>[2x]MASATIPAPAPRKMERAEGPASVLAIG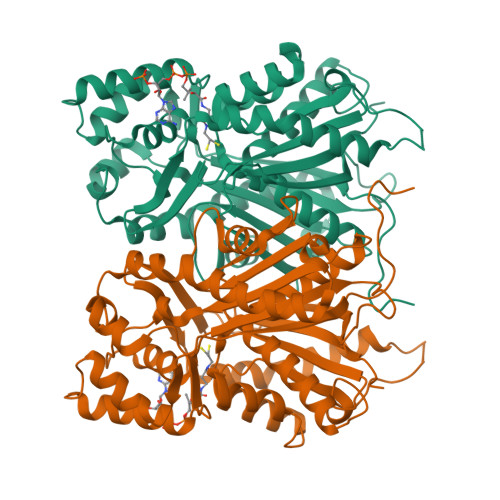TAVPPNVVYQKDYPDFYFGVTNSNHKTELKDKFQRMCDKSCVSKRHLYLTEEILKANPSLCAYWEPSLDLRQDIVVVEVPKLGKQAASAAIKEWGQPKSKITHLIFCTTSGVDMPGADWALAKLLGLRSSVKRLVLYMQGCYGGGTVLRIAKDLAENNKGARVLVVCSEITAITFRGPSDTHLDSLVGQALFGDGASALIVGSDPVPAVERAWFELHWTGSDILPNSDGAIDGHLKEVGLTFHLMKDVPAIISKNIGGILKDALAKVFPAAHDQLDSSGTTAAAPPPPTYNDLFWITHPGGPAILDQVEDRLGLRKDKLASTRAVLDQFGNMSSATVLFIMDEMRKRSVEQQLGTTGEGHEWGLLLGFGPGLTCETVVLRSVPLV> GRGTKSIPPI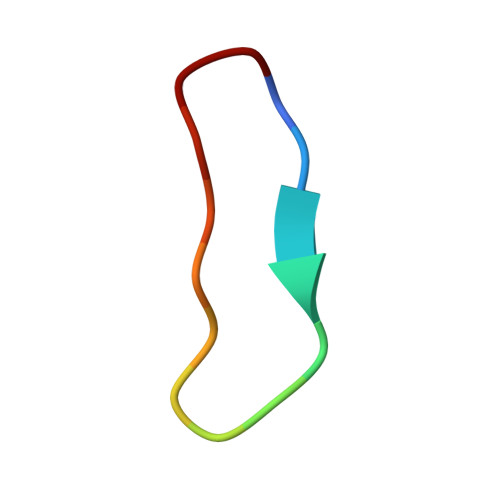AFPD>[2x]GEYK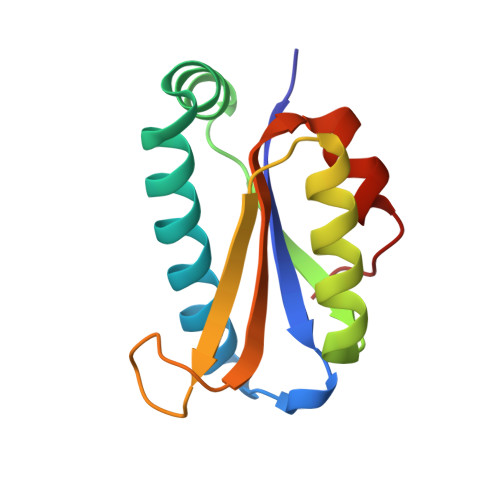MILVVRNDLKMGKGKVAAQCSHAAVSAYKQIQRRNPEMLKQWEYCGQPKVVVKAPDEETLIALLAHAKMLGLTVSLIQDAGRTQIAPGSQTVLGIGPGPADLIDKVTGHLKLY> MLPRPSGTYAGLPIADYGDAPPLSTKTMFWRTSPEKLPPGAWEPAYLGSKDERVDGPSLQQVMRDQLKPYSEPRGLLPPQEILDAVCDAIENRLENTLEPQKPWTFKKACESLDKNTSSGYPYHKQKSKDWTGSAFIGDLGDQATHANNMYEMGKSMRPIYTAALKDELVKPDKIYGKIKKRLLWGSDLGTMIRAARAFGPFCDALKE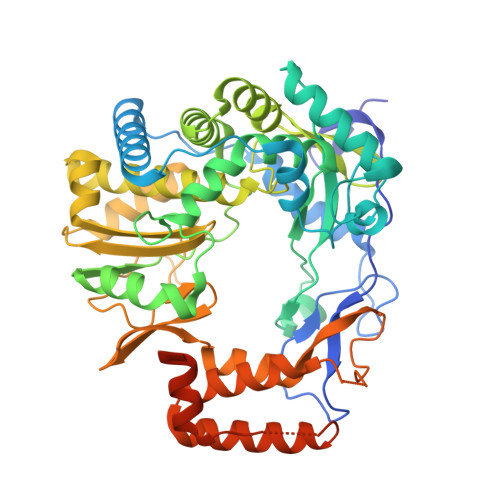TCIFNPIRVGMSMNEDGPFIFARHANFRYHMDADYTRWDSTQQRAILKRAGDIMVRLSPEPDLARVVMDDLLAPSLLDVGDYKIVVEEGLPSGCPCTTQLNSLAHWILTLCAMVEVTRVDPDIVMQESEFSFYGDDEVVSTNLELDMVKYTMALRRYGLLPTRADKEEGPLERRQTLQGISFLRRAIVGDQFGWYGRLDRASIDRQLLWTKGPNHQNPFETLPGHAQRPSQLMALLGEAAMHGEKYYRTVASRVSKEAAQSGIEMVVPRHRSVLRWVRFGTMDAETPQERSAVFVNEDAAALEHHHHHH>MEKDLQLRVNEKLDVENILKDLDKYTPKRRGWTWRQPAENLQMGPFIYKDASTPLENSVALPSAKYFGDIDPQPLPVITTEIASGRFEDDIRRMRMAAWHGADHIMVIRTAGQSHYDGLIEGTPQGIGGVPITRKQVRAQRKALDLIEEEVGRPINYHSYVSGVAGPDIAVMFAEEGVNGAHQDPQYNVLYRNINMIRSFIDACESKTIMAWADMAQIDGAHNANATAREAWKVMPELMVQHALNSIFSLKVGMKKSNICLSTVPPTAPPAPSMYLDLPYAVALREMFEGYRMRAQMNTKYMEASTREATVTHVLNLLISKLTRADIQSTITPDEGRNVPWHIYNIEACDTAKQALIGMDGLMDMVQLKREGVLGDTVRELKERAVLFMEEIIEAGGYFNAVEQGFFVDSGYYPERNGDGIARQINGGIGAGTVFERDEDYMAPVTAHFGYNNVKQYDEALVSEPSKLIDGCTLEVPEKIVYIDELDENDNVNVRMEETKEFRHSSMIKPEVEWQADGTVLLTMFLPTSKRVAEFAAIEFAKKMNLEEVEVINREVMQEAEGTRIELKGRVPFSIDINSLVIPPEPEILSEDEIREDIEKTPLKIVAATVGEDEHSVGLREVIDIKHGGIEKYGVEVHYLGTSVPVEKLVDAAIELKADAILASTIISHDDIHYKNMKRIHELAVEKGIRDKIMIGCGGTQVTPEVAVKQGVDAGFGRGSKGIHVATF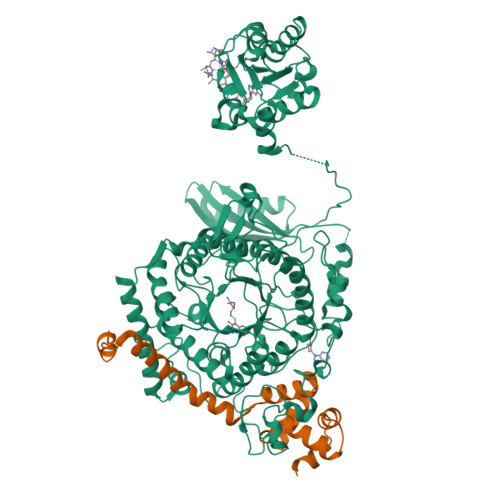LVKKRREMREGKSEDPNSSSVDKLAAALEHHHHHH[4x];>MKRADDFQQRRAHLANLSDEELQTRFWEMAEKIVDPLLDLGKKNTTPSIERSVLLRMGFSSLEAKAIVDKTMDRGLMGKGAGHIVYKIAKEKNISVREAGLALSEGKYWDDAIQIFKGGVK[4x]>MGSINLRIDDELKARSYAALEKMGVTPSEALRLMLEYIADNERLPFKQTLLSDEDAELVEIVKERLRNPKPVRVTLDEL[3x];>MAYFLDFDERALKEWRKLGSTVREQLKKKLVEVLESPRIEANKLRGMPDCYKIK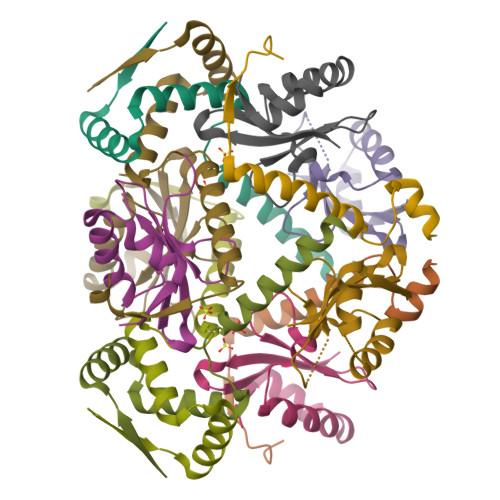LRSSGYRLVYQVIDEKVVVFVISVGKAERSEVYSEAVKRIL[3x]>NGNSLSAAELTCGMIMCLARQIPQATASMKDGKWERKKFMGTELNGKTLGILGLGRIGREVATRMQSFGMKTIGYDPIISPEVSASFGVQQLPLEEIWPLCDFITVHTPLLPSTTGLLNDNTFAQCKK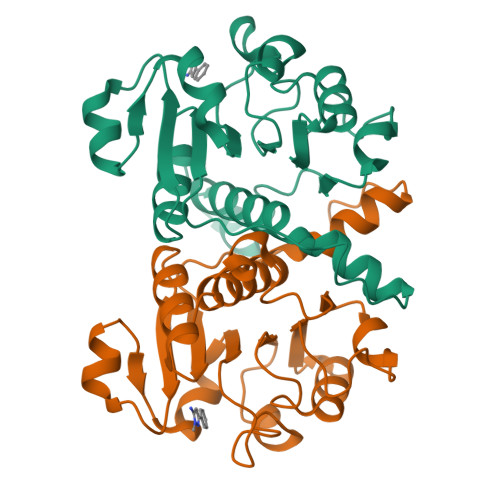GVRVVNCARGGIVDEGALLRALQSGQCAGAALDVFTEEPPRDRALVDHENVISCPHLGASTKEAQSR[2x]>GMTGLSQSQASPMQIQP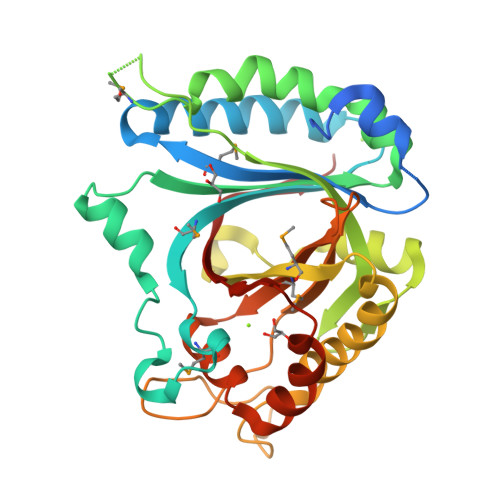GNAAFNPWTDAALDTIRDVNQALTLYAEMRVVPAHHDAFLAAIDTVSAKLRVLPGFLSLALKQMSGDSTMVKNYPETYKGVLATAYLDGVAAGTQPYFYNLFVRFADGRAARAAGFEALFETHIHPLLHAMAPRGGDGPELLAYRAVLQSVVAGDRHAIYRGAEEIRSFLRRPVELPERETVTVENHVMVPEDKHAAWEPQVAILLQVAQDTFEPQDEPSGVGLPGARDNRYYRKALSTEILRNAHADGGLRAYIMHGVWESVWDHENSHLDPRFLAAAGPVGAAAVVGPVEPFYLTRRLVVAD[4x]>[2x]GAMDRVPIMYPIGQMHGTYILAQNENGLYIIDQHAAQERIKYEYFREKVGEVEPEVQEMIVPLTFHY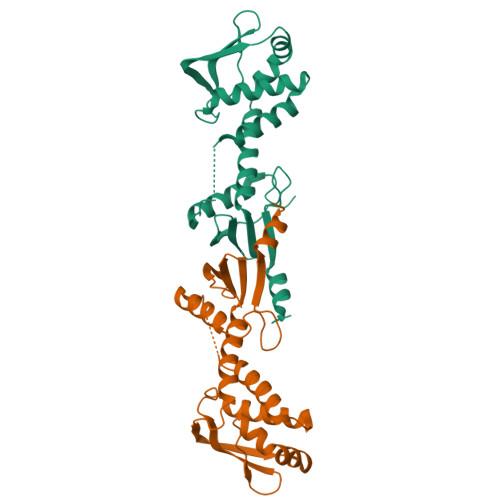STNEALIIEQHKQELESVGVFLESFGSNSYIVRCHPAWFPKGEEAELIEEIIQQVLDSKNIDIKKLREEAAIMMSCKGSIKANRHLRNDEIKALLDDLRSTSDPFTCPHGRPIIIHHSTYEMEKMFKRVM> HHHHHHMNSNRTPSQKVLARQEKIKAVALELFLTKGYQETSLSDIIKLSGGSYSNIYDGFKSKEGLFFEILDDICKKHFHLIY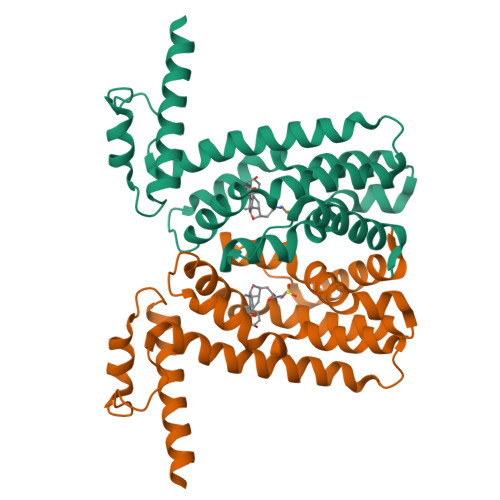SKTQEIKNGTLKEILTSFGLAFIEIFNQPEAVAFGKIIYSQVYDKDRHLANWIENNQQNFSYNILMGFFKQQNNSYMKKNAEKLAVLFCTMLKEPYHHLNVLINAPLKNKKEQKEHVEFVVNVFLNGINSSKA PgcA has been shown to play an important role in EET but is unusual in containing three CXXCH heme binding motifs that are separated by repeated (PT)x motifs, suggested to enhance binding to mineral surfaces. The amino acid sequence of PgcA contains a cleavable Sec signal peptide followed by an N‐terminal lipid anchor and four domains interspersed by repeated (PT)x motifs. The first domain is not predicted to contain any cofactors, while the other three domains are monoheme domains (Fernandes et al., 2023). Furthermore, we demonstrate a distinct role for its domain III as a mineral reductase that is recharged by domains I and II. These findings show PgcA to be the first of a new class of electron transfer proteins, with redox centers separated by some nanometers but tethered together by flexible linkers, facilitating electron transfer through a tethered diffusion mechanism rather than a fixed, closely packed electron transfer chain.

The 1.9 Å crystal structure of heme domain III was composed of PgcA residues 444–511 and is significantly different from those of domains I and II. First, the coordination of the iron atom within the c‐type heme is bis‐His (His459 and His491), as commonly observed in multiheme cytochromes. Second, no acidic side chain is observed near the distal ligating histidine residue. Domain III contains only three α‐helices despite its molecular weight being ~1 kDa larger than those of the preceding two domains. In fact, a greater fraction of its polypeptide chain forms loops that likely possess greater flexibility when unrestricted by crystallization. This crystal structure also shows that 33% of the total surface area of the c‐type heme moiety is solvent exposed, which is substantially larger than the 25% exposure of the hemes in domains I and II. The domain III spectrum is a small g max, rhombic type LS signal (g max 3.08) typical of bis‐histidine coordinated hemes with near parallel ligand orientation. Domains I and II specifically displayed much greater pH dependence, while domain III only shifted by ~10 mV, which is surprising considering the higher solvent accessibility of the domain III heme. We observed that triheme PgcA and domain III bind to akageneite with similar affinity, while neither domains I or II bind at all. While these experiments cannot distinguish between inter‐ and intra‐PgcA electron transfer pathways, these observations show clearly that domain III directly reduces iron(III) oxides, while domains I and II are able to recharge domain III for further electron transfer.

>[2x]MKFKLNLITLALLANTGLAVAADGVDPGKTVYDSRCASCHRLGTYDASGSAPNLSRAGTKIDGKFTAGVSGHKGITLTAADLANLKTFVNANGSGWSHPQFEK> RSPWEGTLPAFLPCELQPHGQVDCNWLFLKSVPHFSAGAPRANVTSLSLISNRIHHLHDSDFVHLSNLRVLNLKWNCPPAGLSPMHFPCRMTIEPNTFLAVPTLEELNLSYNGITTVPALPSSLVSLSLSHTSILVLGPTHFTGLHALRFLYMDGNCYYMNPCPRALEVAPGALLGLGNLTHLSLKYNNLTEVPRRLPPSLDTLLLSYNHIVTLAPEDLANLTALRVLDVGGNCRRCDHARNPCRECPKNFPKLHPDTFSHLSRLEGLVLKDSSLYKLEKDWFRGLGRLQVLDLSENFLYDYITKTTIFNDLTQLRRLNLSFNYHKKVSFAHLHLASSFGSLVSLEKLDMHGIFFRSLTNITLQSLTRLPKLQSLHLQLNFINQAQLSIFGAFPSLLFVDLSDNRISGAATPAAALGEVDSRVEVWRLPRGLAPGPLDAVSSKDFMPSCNLNFTLDLSRNNLVTIQQEMFTRLSRLQCLRLSHNSISQAVNGSQFVPLTSLRVLDLSHNKLDLYHGRSFTELPQLEALDLSYNSQPFSMQGVGHNLSFVAQLPSLRYLSLAHNGIHSRVSQKLSSASLRALDFSGNSLSQMWAEGDLYLCFFKGLRNLVQLDLSENHLHTLL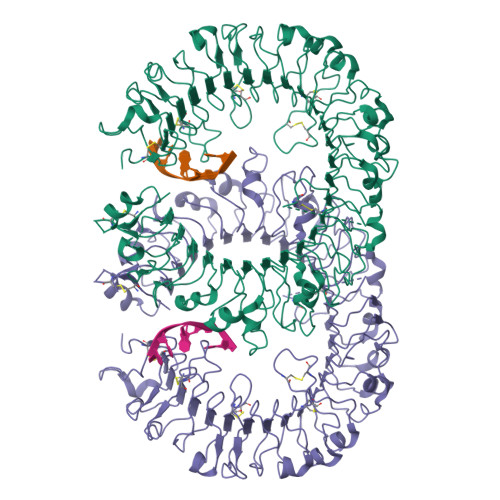PRHLDNLPKSLRQLRLRDNNLAFFNWSSLTVLPRLEALDLAGNQLKALSNGSLPPGIRLQKLDVSSNSIGFVIPGFFVRATRLIELNLSANALKTVDPSWFGSLAGTLKILDVSANPLHCACGAAFVDFLLERQEAVPGLSRRVTCGSPGQLQGRSIFTQDLRLCLDETLSLDEFLVPR> GPHMSSTCTKVLYF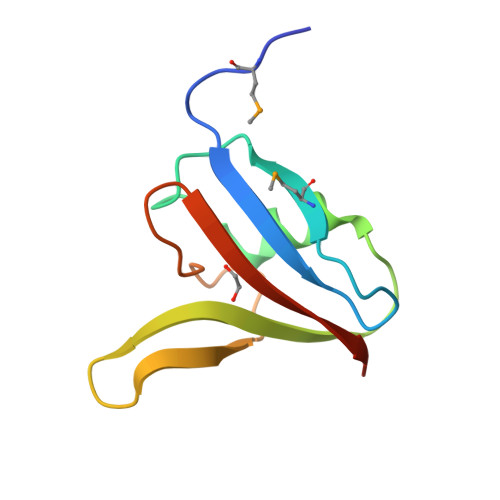TDRSLTPFMVNIPKRLEEVTLKDFKAAIDREGNHRYHFKAMDPEFGTVKEEIFHDDDAIPGWEGKIVAWVEEDHGEN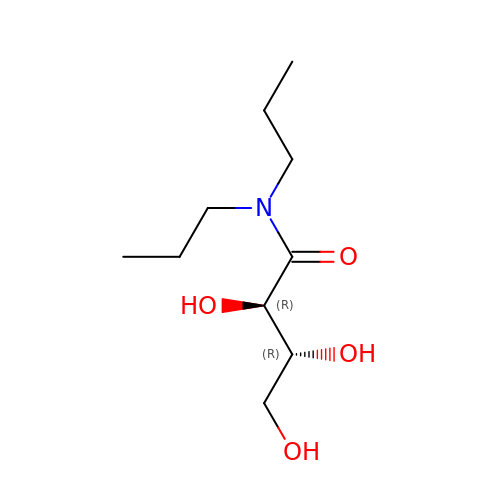(2R,3R)-2,3,4-TRIHYDROXY-N,N-DIPROPYLBUTANAMIDE | C10 H21 N O4 | JYHQCIGUBKFYNN-RKDXNWHRSA-N>SEQLVPIRLEFDQDRDRFFLRDTLLWNKNDKLIKIEDFVDDMLRDYRFEDATREQHIDTICQSIQEQIQEFQGNPYIELNQDRLGGDDLRIRIKLDIVVGQNQLIDQFEWDISNSDNCPEEFAESMCQELELPGEFVTAIAHSIREQVHMYHKSLALLGYNFDGSAIEDDDIRSRMLPTITLDDVYRPAAESK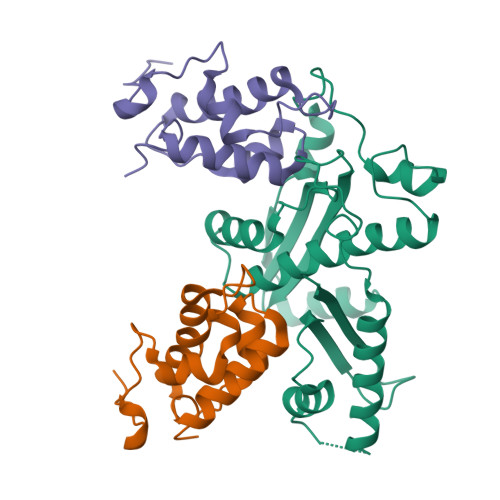IFTPNLLQISAAELERLDKDKDRDTRRKRRQGRS[4x];>DNSIFGDTKSESKQLGNTSSVANTPSEIPDAHKAEQEDIIEKTESVDKKVDSGEERNEQEREIMNDHSKSANPKKTTITRVEPETFEIPQAHEIVIPSYSKWFNLEKIHSIEVQSLPEFFTNRIPSKTPEVYMRYRNFMVNSYRLNPNEYFSVTTARRNVSGDAAALFRLHKFLTKWGLINYQVDSK[8x]>AADEPQLLHGAGICKWFNVRMGFGFLSMTARAGVALDPPVDVFVHQSKLHMEGFRSLKEGEAVEFTFKKSAKGLESIRVTGPGGVFCIGSERRPKGGDRCYNCGGLDHHAKECKLPPQPKKCHFCQSINHMVASCPLKAQ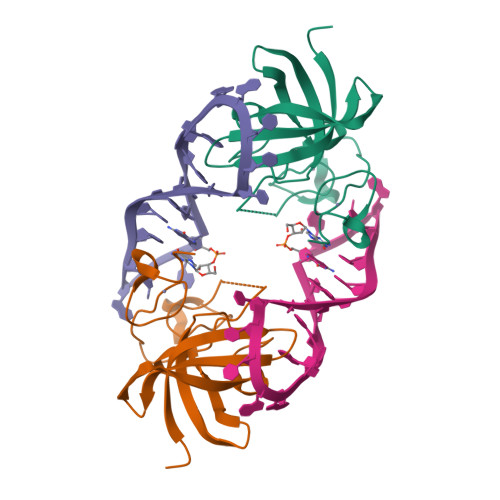QGPSSQGK[6x]> GMSFLFSSRSSKTFKPKKNIPEGSHQYELLKHAEATLGSGNLRQAVMLPEGEDLNEWIAVNTVDFFNQINMLYGTITEFCTEASCPVMSAGPRYEYHWADGTNIKKPIKCSAPKYIDYLMTWVQDQLDD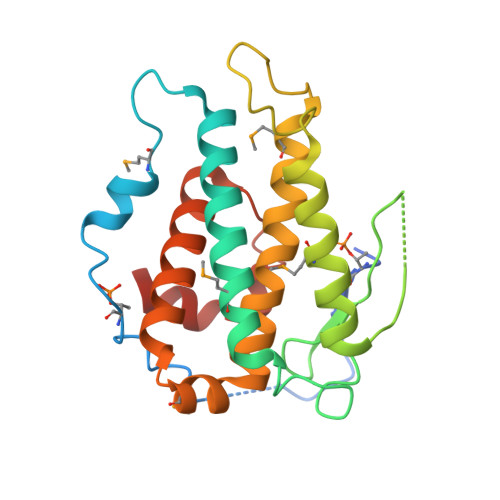ETLFPSKIGVPFPKNFMSVAKTILKRLFRVYAHIYHQHFDSVMQLQEEAHLNTSFKHFIFFVQEFNLIDRRELAPLQELIEKLGSKDR> MADTQYILPNDIGVSSLDCREAFRLLSPTERLYAYHLSRAAWYGGLAVLLQTSPEAPYIYALLSRLFRAQDPDQLRQHALAEGLTEEEYQAFLVYAAGVYSNMGNYKSFGDTKFVPNLPKEKLERVILGSEAAQQHPEEVRGLWQTCGELMFSLEPRLRHLGLGKEGITTYFSGNCTMEDAKLAQDFLDSQNLSAYNTRLFKEVDGEGKPYYEVRLASVLGSEPSLDSEVTSKLKSYEFRGSPFQVTRGDYAPILQKVVEQLEKAKAYAANSHQGQMLAQYIESFTQGSIEAHKRGSRFWIQDKGPIVESYIGFIESYRDPFGSRGEFEGFVAVVNKAMSAKFERLVASAEQ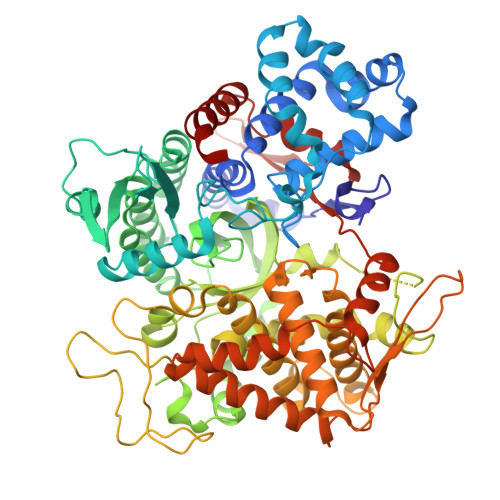LLKELPWPPTFEKDKFLTPDFTSLDVLTFAGSGIPAGINIPNYDDLRQTEGFKNVSLGNVLAVAYATQREKLTFLEEDDKDLYILWKGPSFDVQVGLHALLGHGSGKLFVQDEKGAFNFDQETVINPETGEQIQSWYRSGETWDSKFSTIASSYEECRAESVGLYLCLHPQVLEIFGFEGADAEDVIYVNWLNMVRAGLLALEFYTPEAFNWRQAHMQARFVILRVLLEAGEGLVTITPTTGSDGRPDARVRLDRSKIRSVGKPALERFLRRLQVLKSTGDVAGGRALYEGYATVTDAPPECFLTLRDTVLLRKESRKLIVQPNTRLEGSDVQLLEYEASAAGLIRSFSERFPEDGPELEEILTQLATADARFW> MNILKHFPSYVGPSKIRTLVIPIGHWTRKEFNNAVQKLSEFNEIHLSDVTPIDSPIFTPQGFPHGKLFFDFLTIDHDDALELFLYDFEPFRKTFVIIGLVNDYSDPLTNLNFMKEKYPTLISPNLVYASSTPTKELEQTIDTMENVFASSPDMQKNIETIMCDIARNFLTALNSYYSSYKHVTLRSPGAIGGNAVLKTTLIRQNSYTSSSSSTPMSAVQSSVSSSSKAGSVTTASKRLSSFEMTTNSLKRSASLKLATTLSTSENRSQQKSLGRQMKILGNFQLLAGRYVDALNSFVDAITTLYKVRDYLWLGSALDGISICFLLLSYLGLSYQIPQIVSLICPVEKLNFESSSTGISPVDSNSKATASTTASSTPRNSISIAAMQSPRNSIMSLSAPALNIDVENINLPLLIKCISDKVLYYYDLSLMHNSEYAPQVVYCEFLLKTLTFMTSCYKSSEFSKDVLDNIVKNQHRALSDIPNSPMFPRFEVYFYSNKLFELQLKEMQVEAQIKIYSTMAEVYRLLGYKRKQLFVLRLLMVALLATPNKIAWHP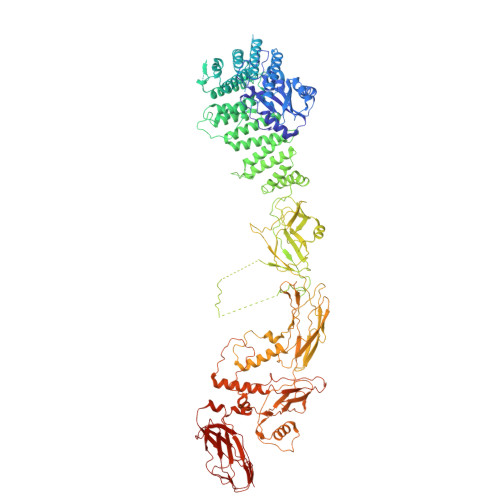DYRTLIDTIIELLNINESEAKINVDDPSQSTWLILQKKILQLCIKVSRKINDFEYVAKFSSILITKYTHLLNQSEQDALFKEYIQPSITNESITSYWDPFILREVVINRILDSDPTSNEIPLESDVSSLESLENRQKTQDINPQEVFNPFKRVQPTSFVSNNSTKVPILVFLVGDKAEFTCRVQNPFKFDFTINDIQLDEEISEFCEIDRKAVSYSGPYNVKAESIRSITLPLIIKKPTYKKIYEISCLKISILKLPLQKFDIINDSRRSNPVEEEAEYSKCIYGKLKIKILPEQPQLELLSTSKMTRNSWMMLDGTKTDFHITVRNKSLSCAINHIKIIPMNNIEQMLKPDYWKKMPPDDLYIMEKQLDWLSKSCVRIIKLPTVIKPNETITFDLELDNTAVPFNFTGFDLLIEYGMSATDESCIYLKKLSIPYEVTLRRTIEVPSMDIIPLNELFSSQVENVDWIEYVMSKIRAESNLHSRDFILLLLDFRNSWIDGIKLNVQFEDFTSNEYHVEASHTSRIIVPIKKIDYKKYNFENTPIPRIYPGRQFIQSGLNEEQTIEMRQKFWCREHIISKLKCNWKLTTDQSVTGSVDFNKFIEKFDHKMVYTIYPGRLFYGVQLLLDEPKVKVGEIINLKIITEPTSTCRRKQNSTVNFLDIVIFDSKTSKILPRSNRRILYNGSLTKPISTTKVSEINLEIIPIEKGRYEFSVCISKSNNQDGIIQFDSENVILSVI> NGKSQSIIV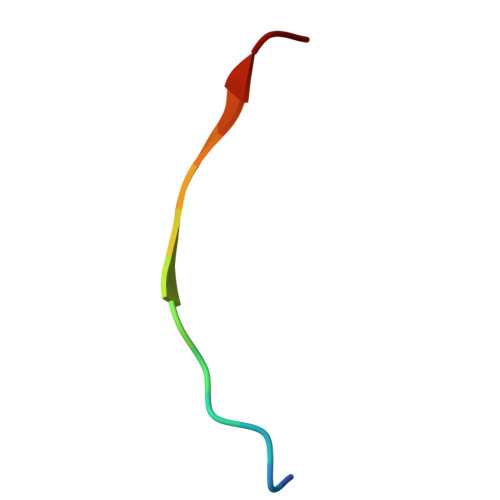GPWGD>GSKFSAKRLPSTRLGTFLENRVNDFLRRQNHPESGEVTVRVVHASDKTVEVKPGMKARFVDSGEMAESFPYRTKALFAFEEIDGVDLCFFGMHVQEYGSDCPPPNQRRVYISYLDSVHFFRPKCLRTAVYHEILIGYLEYVKKLGYTTGHIWACPPSEGDDYIFHCHPPDQKIPKPKRLQEWFKKMLDKAVSERIVHDYKDIFKQATEDRLTSAKELPYFEGDFWPNVLEESIKESGGSGSQKLYATMEKHKEVFFVIRLIA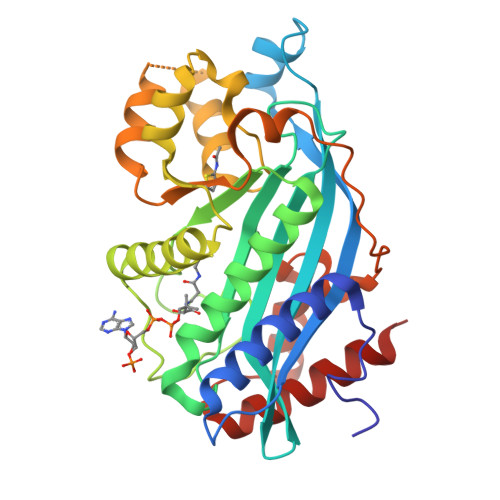GPAANSLPPIVDPDPLIPCDLMDGRDAFLTLARDKHLEFSSLRRAQWSTMCMLVELHTQSQ[2x]1-benzyl-1,4,5,6-tetrahydropyridine-3-carboxamide | C13 H16 N2 O | 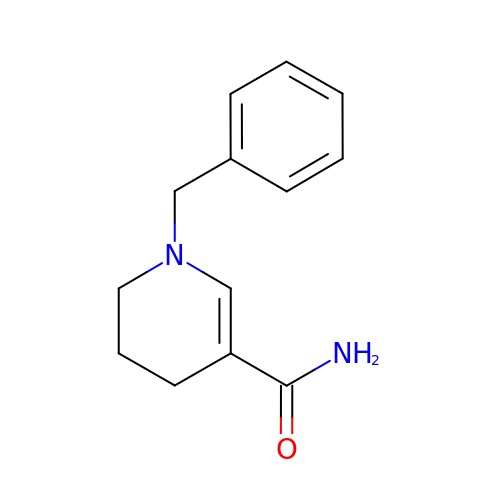MSZLGNZPMBNYEO-UHFFFAOYSA-N(2R,3R,4R,5R,6R)-5-acetamido-6-[(1R,2R)-1,2-bis(oxidanyl)propyl]-2,3-bis(fluoranyl)-4-oxidanyl-oxane-2-carboxylic 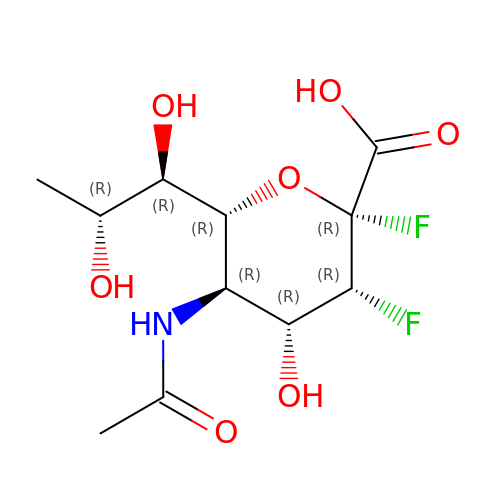acid | C11 H17 F2 N O7 | PRVRMQAFLBOHCL-GEFXCWNQSA-N>[3x]MLYLTQRLEIPAAATASVTLPIDVRVKSRVKVTLNDGRDAGLLLPRGLLLRGGDVLSNEEGTEFVQVIAADEEVSVVRCDDPFMLAKACYALGNRHVPLQIMPGELRYHHDHVLDDMLRQFGLTVTFGQLPFEPEAGAYASES;> MLYLTQRLEIPAAATASVTLPIDVRVKSRVKVTLNDGRDAGLLLPRGLLLRGGDV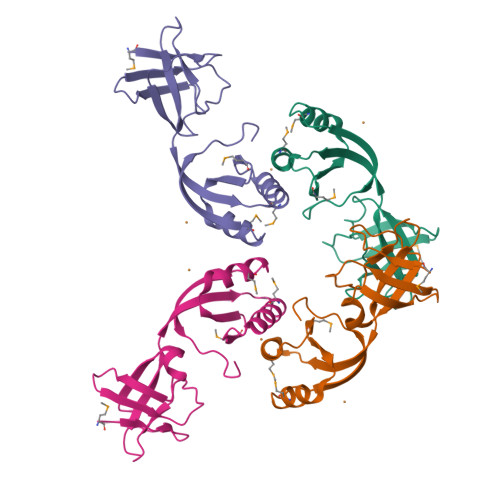LSNEEGTDFVQVIAADEEVSVVRCDDPFMLAKACYALGNRHVPLQIMPGELRYHHDHVLDDMLRQFGLTVTFGQLPFEPEAGAYASES1-O-phosphono-beta-D-fructopyranose | 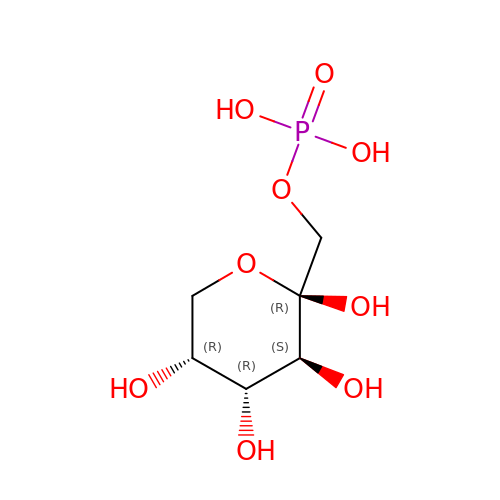C6 H13 O9 P | HXRNACQBNUPKDX-ARQDHWQXSA-N>AHSDASSDITLKVAIYPYVPDPARFQAAVLDQWQRQEPGVKLEFTDWDSYSADPPDDLDVFVLDSIFLSHFVDAGYLLPFGSQDIDQAEDVLPFALQGAKRNGEVYGLPQILCTNLLFYRKGDLKIGQVDNIYELYKKIGTSHSEQIPPPQNKGLLINMAGGTTKASMYLEALIDVTGQYTEYDLLPPLDPLNDKVIRGLRLLINMAGEKPSQYVPEDGDAYVRASWFAQGSGRAFIGYSESMMRMGDYAEQVRFKPISSSAGQDIPLFYSDVVSVNSKTAHPELAKKLANVMASADTVEQALRPQADGQYPQYLLPARHQVYEALMQDYPIYSELAQIVNKPSNRVFRLG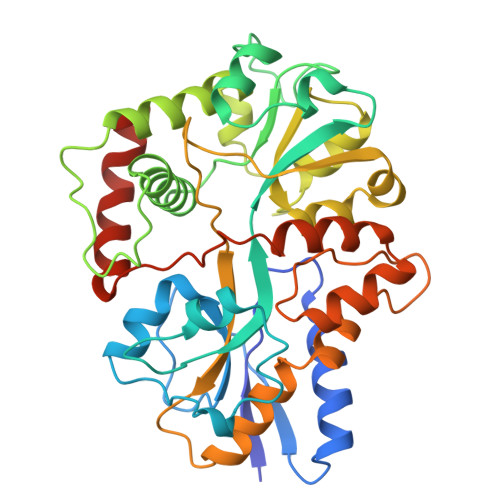PEVRTWLKDAKQVLPEALGLTDVSSLAS[2x]pyridazin-3-amine | C4 H5 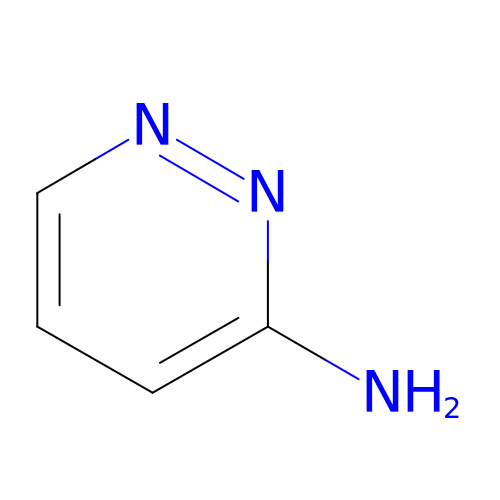N3 | LETVJWLLIMJADE-UHFFFAOYSA-N> GAKPRNLNVSFQGCGMDSLSVRAMDTDTLTQVKEKILEAFCKNVPYSQWPRAEDVDLEWFASSTQSYILRDLDDTSVVEDGRKKLNTLAHYKIPEGASLAMSLIDKKDNTLGR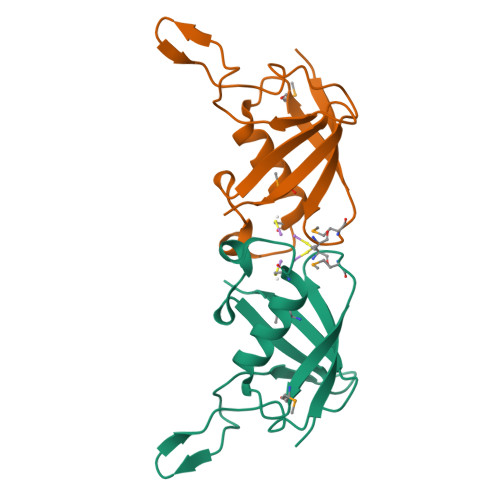VKDLDTEKYFHLVL>MGSHHHHHHSSGLVPRGSHMELHILEHRVRVLSVARPGLWLYTHPLIKLLFLPRRSRCKFFSLTETPEDYTLMVDEEGFKELPPSEFLQVAEATWLVLNVSSHSGAAVQAAGVTKIARSVIAPLAEHHVSVLMLSTYQTDFILVREQDLSVVIHTLAQEFDIYREVGGEPVPVTRDDSSNGFPRTQHGPSPTVHPIQSPQNRFCVLTLDPETLPAIATTLIDVLFYSHSTPKEAASSSPEPSSITFFAFSLIEGYISIVMDAETQKKFPSDLLLTSSSGELWRMVRIGGQPLGFDECGIVAQIAGPLAAADIS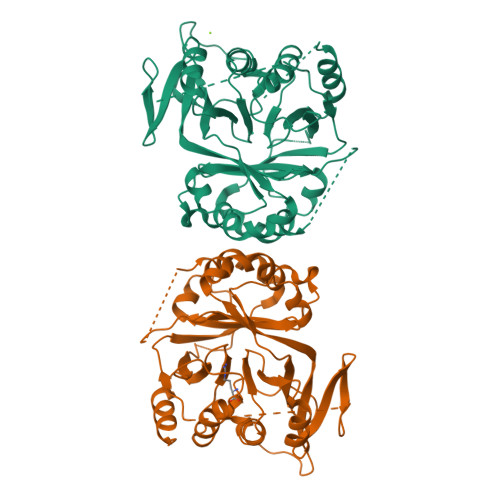AYYISTFNFDHALVPEDGIGSVIEVLQRRQEGLASR[2x]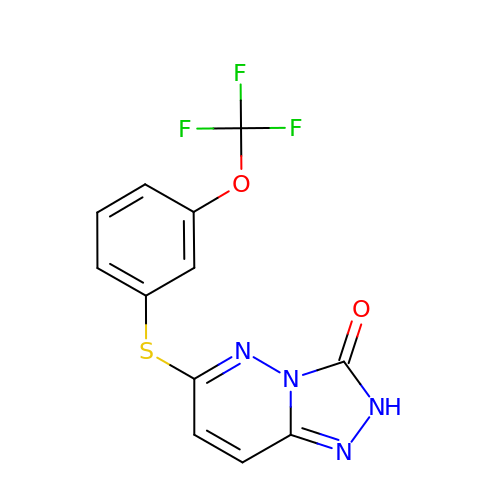6-((3-(trifluoromethoxy)phenyl)thio)-[1,2,4]triazolo[4,3-b]pyridazin-3(2H)-one | C12 H7 F3 N4 O2 S | SFULZVNQBHXFMN-UHFFFAOYSA-N> STAFFFRRMSPADK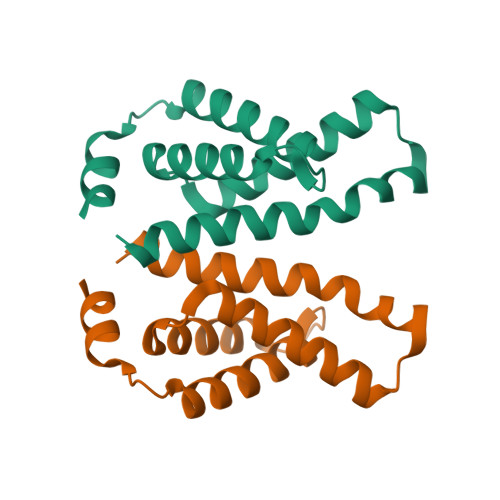RKLLDELRSIYRTIVLEYFNTDAKVNERIDEFVSKAFFADISVSQVLEIHVELMDTFSKQLKLEGRSEDILLDYRLTLIDVIAHLCEMYRRSIPREV(3~{Z})-4-methyl-3-(phenylmethylidene)-1~{H}-1,4-benzodiazepine-2,5-dione 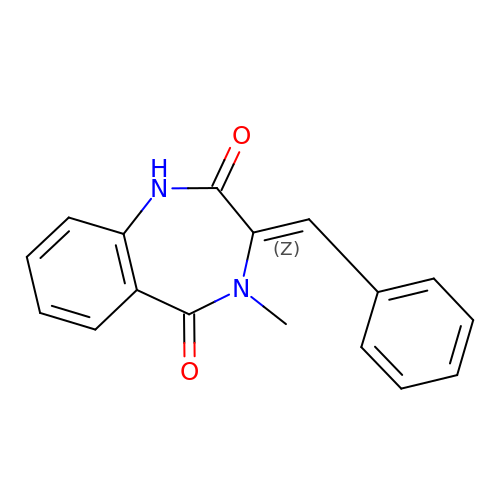| C17 H14 N2 O2 | FYVKHLSOIIPVEH-PTNGSMBKSA-N>[2x]MEQRITLKDYAMRFGQTKTAKDLGVYPSSINQAIHAGRKIFLTINADGSVYAEEVKPF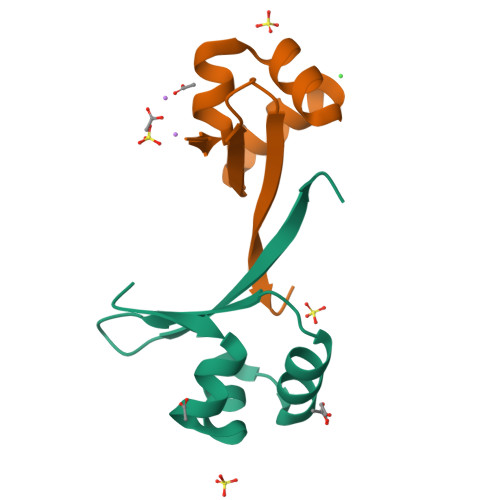PSNKKTTA> MYLTKEEELILAGEYGYALQKAMEILVALGDIYGADRLIPIKSAQVAGVSYKNIGDAGIEFLRDFVEAGAKVSVYTTLNPAGIGDDEFMEKQMEVLELYRKMGIEVTSTCTPYYGAN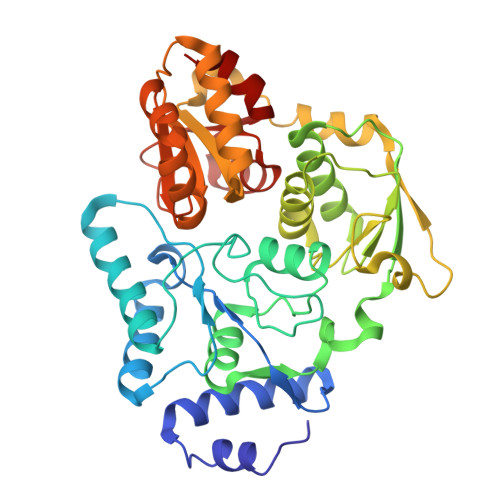LPKFGDHIAWSESSAVSFANSILGARTNREGGPSSLAAAIVGKTPNYGLHLDENRKATVIVDVKAKVKTFADYSVLGYHVGKTLGNDVPYFKNLKPEKTEFLKELGAAMGATGSIALYHVEGETPEYREAITDKLETITVEDSDLKAVRESFQDDWSDIDMILIGCPHASLPEVKEIAELLRMRGKPLKIPLFITASRAVKALADALGYTEIIERYNGKIIPDSCFVVSPIKGWYRGIATNSGKSAFYFRSFGFSVRLDDVENLIKEAP~{N}-[4-[5-(3-aminophenyl)-6-(1-methylpyrazol-4-yl)furo[2,3-d]pyrimidin-4-yl]oxyphenyl]-1-(4-fluorophenyl)-2-oxidanylidene-pyridine-3-carboxamide | C34 H24 F N7 O4 | 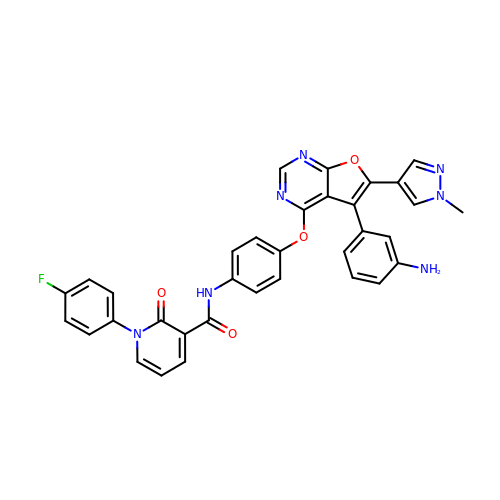NCGOROUZONSZHC-UHFFFAOYSA-N> MGSSHHHHHHSSGENLYFQIGDEFGDDDRSSMSDDGPRHDADDHGPRGEDRGDDDRGNAPSNGRGPVTGIGTASADELIAIADAARGAADGEVTSIDAKRDGTWEVQLTTAAGAETEVRVDEALVASVTSTDAADGDDTGPALTLDDETIRALVSAALAEAEGMITDLDVDGDDVSPYDASVLTSDNRSIDIDFSADFAVVGTD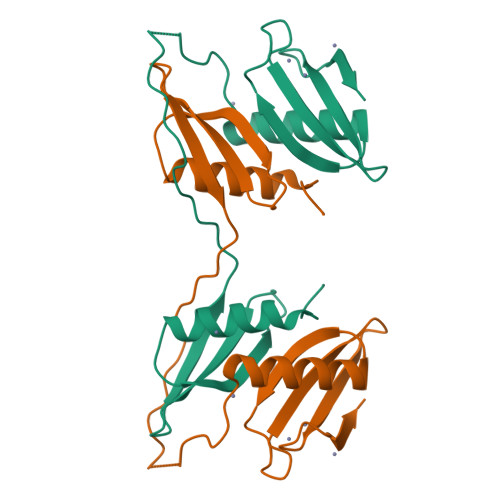ID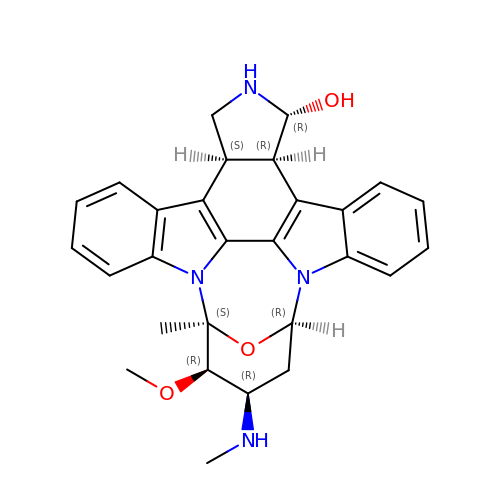(5S,6R,7R,9R,13cR,14R,16aS)-6-methoxy-5-methyl-7-(methylamino)-6,7,8,9,14,15,16,16a-octahydro-5H,13cH-5,9-epoxy-4b,9a,15-triazadibenzo[b,h]cyclonona[1,2,3,4-jkl]cyclopenta[e]-as-indacen-14-ol | C28 H30 N4 O3 | FJJCTPAMIAOFJX-VWKRKTLRSA-N but-2-yn-1-yl trihydrogen diphosphate | C4 H8 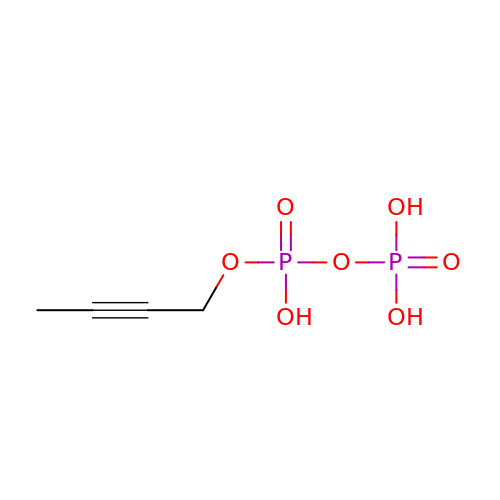O7 P2 | MMKJTWNLJFDOFE-UHFFFAOYSA-N>[2x]ADFEVHMLNKGKDGAYVFEPASL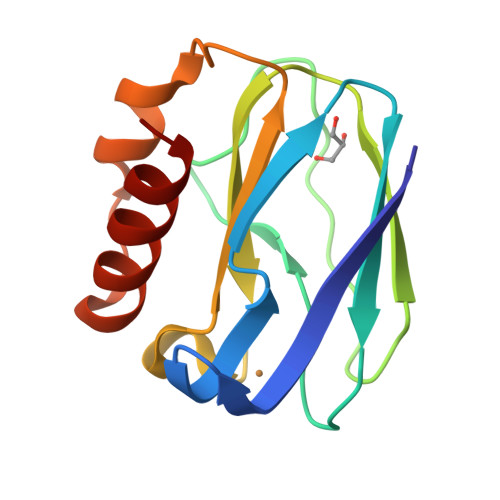KVAPGDTVTFIPTDKGHNVETIKGMIPDGAEAFKSKINENYKVTFTAPGVYGVKCTPHYGMGMVGVVQVGDAPANLEAVKGAKNPKKAQERLDAALAALGN> MGSSHHHHHHHHGASENLYFQGASMTRATNFTELYAGKGILDTYMVAEKITRYYTQDLIQLSGLSESSLTPLVILDLACGTGVVSDALHDMLNFQPKGNWELTCGDISTELTGHVKQKILERG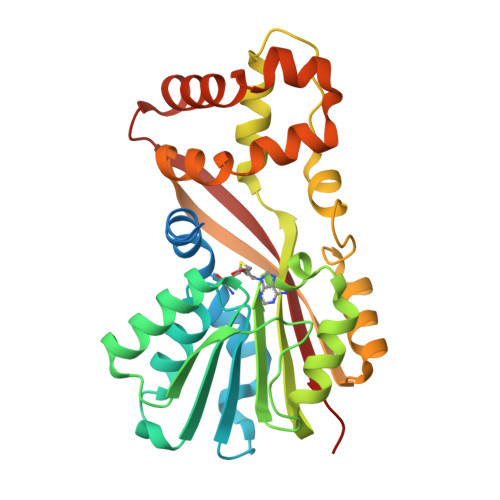WENSIAKVVDAQNTELPTGHYTHVFAALAFTSFPDTYAAMKEVMRILQPGGTLTISTWQRTEWLAVVEAAVAIIPADLPFPTTKEFMSCMNPGWDSEDYVHSRFEEAGFHSVQVTTISKQFETSVEDLYKIAQPVIPIIVSKWWNQEQRDKYENDILPALQRHLNETYGENGLVPQEWTAVFATGQKGS> GPLSMSCWLREQTLLLAEDYISFCSGIQQTP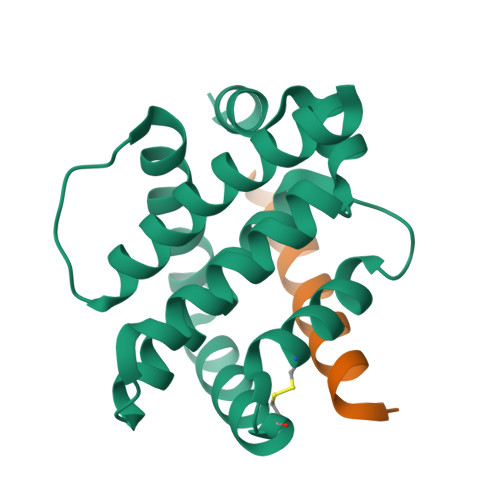PSESAEAMRYLAKEMEQQHRTKFRSLSQEFLDTCGADPSKCLQSVMRELVGDGKMNWGRVVSIFTFTGVLASELLSRGENSEGSRRLAETIADYLGGEKQDWLVENGGWEGFCRFFHNARQ;> ALWAAKKYGQQLRRMSDEFDKGQMKR LysK, an endolysin from staphylococcal phage K, contains an N-terminal cysteine-histidine dependent amido-hydrolase/peptidase domain (CHAPK), a central amidase domain and a C-terminal SH3b cell wall-binding domain. CHAPK cleaves bacterial peptidoglycan between the tetra-peptide stem and the penta-glycine bridge. The structure has the papain-type fold with a long loop between the two amino-terminal alpha-helices. The structure suggests the location of the active site near a hydrophobic groove, with Cys54, His117 and Glu134 forming the catalytic triad.

We determined the structure of the CHAPK domain of LysK at 1.8 Å resolution (1 Å = 0.1 nm). For the native structure, a calcium ion, a zinc ion and a 2-(N-morpholino)ethanesulfonic acid (MES) molecule have been modelled associated with each of the protein chains. Other ordered solvent molecules have also been modelled in the asymmetric unit and consist of one glycerol molecule, four putative sodium ions and 741 water molecules. A calcium ion was found tightly bound to the protein. Its ligands are the side-chains of Asp45, Asp47 and Asp56, plus the backbone oxygens of Tyr49 and His51, all in the amino-terminal domain specific to CHAPK. It likely has a structural role, stabilizing the protein fold. Also, the occupancy appears to be less than unity, we estimate it to be around 0.67 based on refinement runs performed at different occupancies. Finally, the resulting electron density around the zinc ions is somewhat ambiguous and we could not model the ligands without some remaining uncertainty. The coordination distances for the zinc ion are not ideal; the zinc ion is too close to Cys54 and too far from the coordinating oxygen atoms. Zinc ions may play a regulatory role, and their binding near Cys54 suggests they may regulate access of the substrate to the catalytic site.

>[4x]MAKTQAEINKRLDAYAKGTVDSPYRVKKATSYDPSFGVMEAGAIDADGYYHAQCQDLITDYVLWLTDNKVRTWGNAKDQIKQSYGTGFKIHENKPSTVPKKGWIAVFTSGSYEQWGHIGIVYDGGNTSTFTILEQNWNGYANKKPTKRVDNYYGLTHFIEIPVKA>DDACNVNIFDAIAEIGNQLYLFKDGKYWRFSEGRGSRPQGPFLIADKWPALPRKLDSVFEEPLSKKLFFFSGRQVWVYTGASVLGPRRLDKLGLGADVAQVTGALRSGRGKMLLFSGRRLWRFDVKAQMVDPRSASEVDRMFPGVPLDTHDVFQFREKAY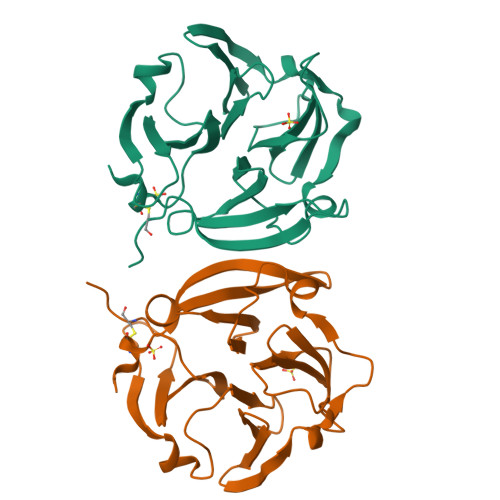FCQDRFYWRVSSRSELNQVDQVGYVTYDILQCPED[2x]>MEQSHQNLQSQFFIEHILQILPHRYPMLLVDRITELQANQKIVAYKNITFNEDVFNGHFPNKPIFPGVLIVEGMAQSGGFLAFTSLWGFDPEIAKTKIVYFMTIDKVKFRIPVTPGDRLEYHLEVLKH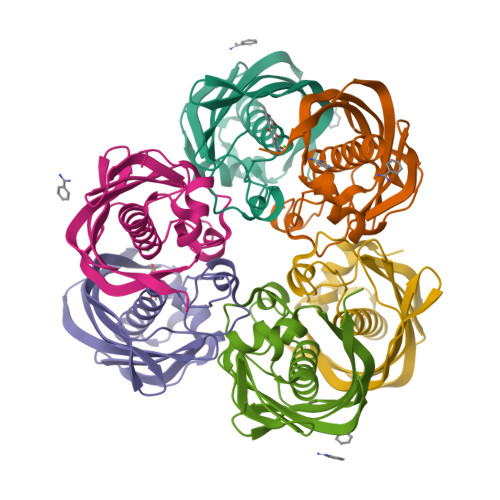KGMIWQVGGTAQVDGKVVAEAELKAMIAERE[6x]>GMSKYKLIMLRHGEGAWNKENRFCSWVDQKLNSEGMEEARNCGKQLKALNFEFDLVFTSVLNRSIHTAWLILEELGQEWVPVESSWRLNERHYGALIGLNREQMALNHGEEQVRLWRRSYNVT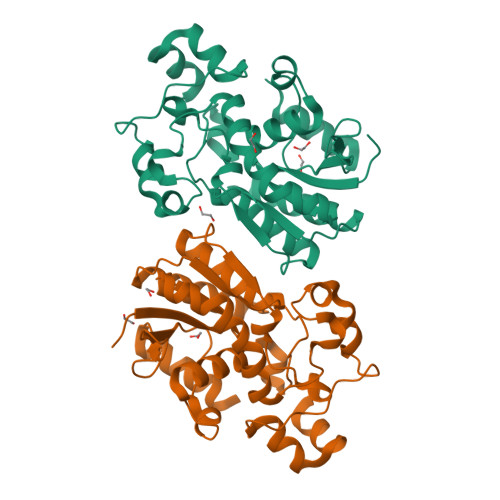PPPIEESHPYYQEIYNDRRYKVCDVPLDQLPRSESLKDVLERLLPYWNERIAPEVLRGKTILISAHGNSSRALLKHLEGISDEDIINITLPTGVPILLELDENLRAVGPHQFLGDQEAIQAAIKKVEDQGKVKQAKK[2x]> MEHQLLCCEVETIRRAYPDANLLNDRVLRAMLKAEETCAPSVSYFKCVQKEVLPSMRKIVATWMLEVCEEQKCEEEVFPLAMNYLDRFLSLEPVKKSRLQLLGATCMFVASKMKETIPLTAEKLCIYTDNSIRPEELLQMELLLVNKLKWNLAAMTPHDFIEHFLSKMPEAEENKQIIRKHAQTFVALCATDV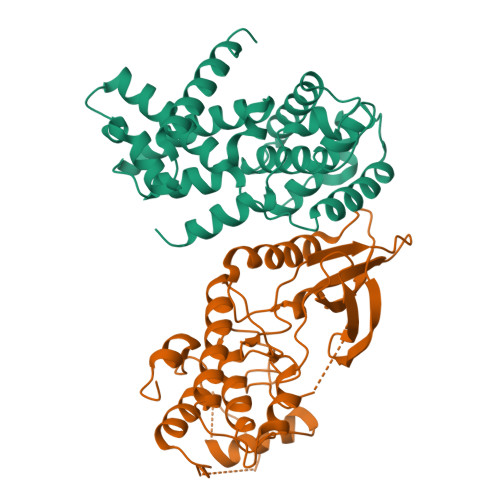KFISNPPSMVAAGSVVAAVQGLNLRSPNNFLSYYRLTRFLSRVIKCDPDCLRACQEQIEALLESSLRQAQQNMDPKAA;> MATSRYEPVAEIGVGAYGTVYKARDPHSGHFVALKSVRVPNGEEGLPISTVREVALLRRLEAFEHPNVVRLMDVCATSRTDREIKVTLVFEHVDQDLRTYLDKAPPPGLPAETIKDLMRQFLRGLDFLHANCIVHRDLKPENILVTSGGTVKLADFGLARIYSYQMALFPVVVTLWYRAPEVLLQSTYATPVDMWSVGCIFAEMFRRKPLFCGNSEADQLGKIFDLIGLPPEDDWPRDVSLPRGAFPPRGPRPVQSVVPEMEESGAQLLLEMLTFNPHKRISAFRALQHSYLHKDEGNPEHHHHHH>[2x]MNHAQLRRVTAESFAHYRHGLAQLLFETVHGGASVGFMA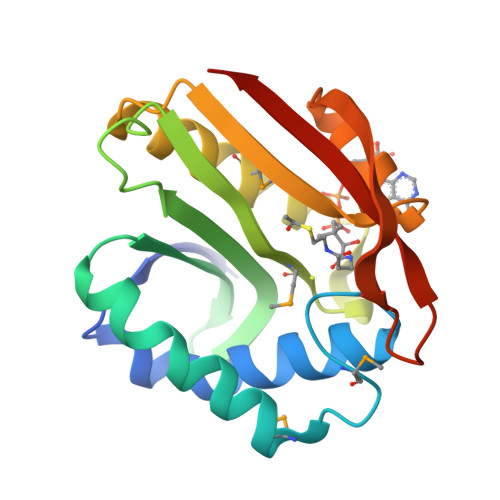DLDMQQAYAWCDGLKADIAAGSLLLWVVAEDDNVLASAQLSLCQKPNGLNRAEVQKLMVLPSARGRGLGRQLMDEVEQVAVKHKRGLLHLDTEAGSVAEAFYSALAYTRVGELPGYCATPDGRLHPTAIYFKTLGQPT>YFQSMLKPYAVDFQRRYKQFSQILKNIGENEGGIDKFSRGYESFGVHRCADGGLYCKEWAPGAEGVFLTGDFNGWNPFSYPYKKLDYGKWELYIPPKQNKSVLVPHGSKLKVVITSKSGEILYRISPWAKYVVREGDNVNYDWIHWDPEHSYEFKHSRPKKPRSLRIYESHVGISSHEGKVASYKHFTCNVLPRIKGLGYNCIQLMAIMEHAYYASFGYQITSFFAASSRYGSPEELQELVDTAHSMGIIVLLDVVHSHASKNSADGLNMFDGTDSCYFHSGPRGTHDLWDSRLFAYSSWEVLRFLLSNIRWWLEEYRFDGFRFDGVTSMLYH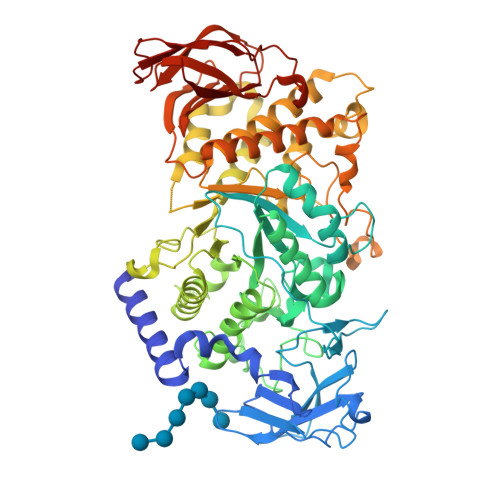HHGVGQGFSGDYSEYFGLQVDEDALTYLMLANHLVHTLCPDSITIAEDVSGMPALCSPISQGGGGFDYRLAMAIPDKWIQLLKEFKDEDWNMGDIVYTLTNRRYLEKCIAYAESHDQALVGDKSLAFWLMDAEMYTNMSVLTPFTPVIDRGIQLHKMIRLITHGLGGEGYLNFMGNEFGHPEWLDFPRKGNNESYHYARRQFHLTDDDLLRYKFLNNFDRDMNRLEERYGWLAAPQAYVSEKHEGNKIIAFERAGLLFIFNFHPSKSYTDYRVGTALPGKFKIVLDSDAAEYGGHQRLDHSTDFFSEAFEHNGRPYSLLVYIPSRVALILQNVDL[3x]>[12x]MATKAARAPRTVLPFEAMPQHPGNRWLRLLQIWREQGYEHLHLEMHQTFQELGPIFRYNLGGPRMVCVMLPEDVEKLQQVDSLHPCRMILEPWVAYRQHRGHKCGVFLLNGPEWRFNRLRLNPDVLSPKAVQRFLPMVDAVARD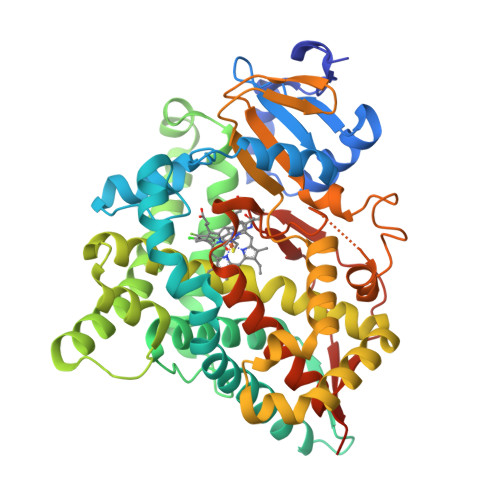FSQALKKKVLQNARGSLTLDVQPSIFHYTIEASNLALFGERLGLVGHSPSSASLNFLHALEVMFKSTVQLMFMPRSLSRWISPKVWKEHFEAWDCIFQYGDNCIQKIYQELAFNRPQHYTGIVAELLLKAELSLEAIKANSMELTAGSVDTTAFPLLMTLFELARNPDVQQILRQESLAAAASISEHPQKATTELPLLRAALKETLRLYPVGLFLERVVSSDLVLQNYHIPAGTLVQVFLYSLGRNAALFPRPERYNPQRWLDIRGSGRNFHHVPFGFGMRQCLGRRLAEAEMLLLLHHVLKHFLVETLTQEDIKMVYSFILRPGTSPLLTFRAINGGRHHHHHH>[2x]C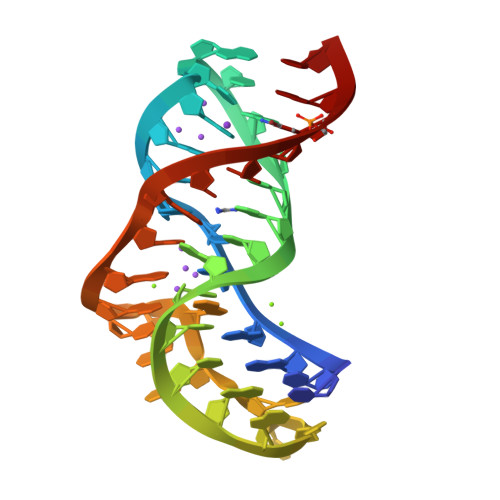CGGACGAGGUGCGCCGUACCCGGUCAGGACAAGACGGCGC>[6x]GAMGASGKIKISTPYNLTKRMMMPMLNGFMSQYPEINIELTTESNADQLDPTEWDVIFRVGP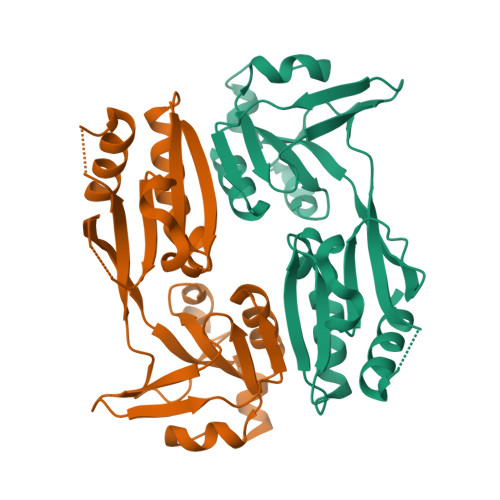QRDSSLIARKIGSVKDILVASPEYVNAHPMPTHAEDLHDHFLLKGHPLLKWTLINSKGETVVNVDRGRFQANALNVVRSACSEGLGITLMPDVMIKEYIADGSLVRILPDWSANPRDIYMLYNHKDHLPEKVRLFIDYVIAYNIH>[10x]MTTSASSHLNKGIKQVYMSLPQGEKVQAMYIWIDGTGEGLRCKTRTLDSEPKCVEELPEWNFDGSSTLQSEGSNSDMYLVPAAMFRDPFRKDPNKLVLCEVFKYNRRPAETNLRHTCKRIMDMVSNQHPWFGMEQEYTLMGTDGHPF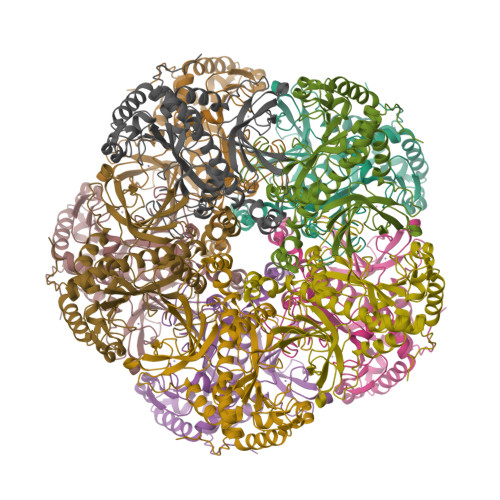GWPSNGFPGPQGPYYCGVGADRAYGRDIVEAHYRACLYAGVKIAGTNAEVMPAQWEFQIGPCEGISMGDHLWVARFILHRVCEDFGVIATFDPKPIPGNWNGAGCHTNFSTKAMREENGLKYIEEAIEKLSKRHQYHIRAYDPKGGLDNARRLTGFHETSNINDFSAGVANRSASIRIPRTVGQEKKGYFEDRRPSANCDPFSVTEALIRTCLLNETGDEPFQYKN>[8x]MFKPHVTVACVVHAEGKFLVVEETINGKALWNQPAGHLEADETLVEAAARELWEETGISAQPQHFIRMHQWIAPDKTPFLRFLFAIELEQICPTQPHDS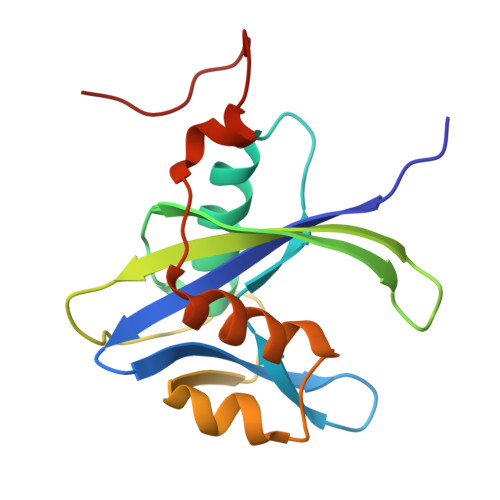DIDCCRWVSAEEILQASNLRSPLVAESIRCYQSGQRYPLEMIGDFNWPFTKGVI>[2x]MGSSHHHHHHSQDPSSMTMELRPSGDSGSSDVDAEISDGFSPLDTSHRDVADEGSLLRRAEMYQDYMKQVPIPTNRGSLIPFTSWVGLSISMKQLYGQPLHYLTNVLLQRWDQSRFGTDSEEQRLDSIIHPTKAEATIWLVEEIHRLTPSHLHMALLWRSDPMYHSFIDPIFPEK;>[4x]MADLYPTGQQISFQTTPLNVQDPTRMMNLDQSSPVARNETQNGGGIAHAEFAMFNSKRLESDLEAMGNKIKQHEDNLKFLKSQKNKMDEAIVDLQVHMSKLNSSPTPRSENSDNSLQGEDINAQILRHENSAAGVLSLVETLHGAQASQLMLTKGVVGVVAKLGKVNDENLSQILSNYLGTRSMLAVVCRNYESVTALEAYDNHGNIDINAGLHCLGSSIGREIGDSFDAICLENLRPYVGQHIADDLQRRLDLLKPKLPNGECPPGFLGFAVNMIQIDPAYLLCVTSYGYGLRETLFYNLFSRLQVYKTRADMISALPCISDGAVSLDGGIIRKTGIFNLGNRDEVNVRFAKPTASRTMDNYSEAEKKMKELKWKKEKTLEDIKREQVLREHAVFNFGKKKEEFVRCLAQSSCTNQPMNTPRGTLESGKETAAAKFERQHMDSSTSAA

RdDM requires two plant-specific RNA polymerases known as RNA polymerase IV (Pol IV) and RNA polymerase V (Pol V), and a number of accessory proteins with different functions. All together, these observations have positioned the DDR complex as a key component that acts downstream of the methylation readers SUVH2/SUVH9 to recruit Pol V to RdDM loci. We report here the structures of the Arabidopsis Pol V recruitment complexes DR (DMS3-RDM1) and DDR′ (DRD1 peptide 7-DMS3-RDM1). The structures of the two complexes are similar at their core—two DMS3 dimers bridged by an RDM1 dimer.

Using single-particle cryoEM, we determined the structure of the DR complex to an overall resolution of 3.6 Å. The cryoEM structure shows that the stoichiometry of DMS3:RDM1 is 4:2. The two RDM1 molecules in the DR complex form a dimer at the center of the complex. Surrounding this RDM1 dimer core are four DMS3 molecules that form two dimers, each binding to the exposed sides of a RDM1 monomer of the dimer core, opposing one another. In addition, the two DMS3 dimers bridge to each other across the RDM1 dimer core using two CC arms. Interestingly, while the two DMS3 dimers are similar to one another, the two monomers within each DMS3 dimer differ in their structures: one shows both visible hinge and CC domains, while the other monomer has a visible hinge but unresolved CC domain in the structure. DMS3 dimerizes using two hinge domains in a hand-shake configuration, forming a donut shape. Our cryoEM structure of the DR complex also reveals numerous interactions between DMS3 dimer and RDM1, with a buried interface with an estimated area of ~31% of the RDM1 dimer surface area. Notably, both pockets are occupied by the CC arm of DMS3 in our cryoEM structure (inset 3). We hypothesize that the DR complex might represent an early intermediary complex prior to the formation of the full DDR complex.>XSAVKAARYGKDNVRVYKVHKDEKTGVQTVYEMTVCVLLEGEIETSYTKADNSVIVATDSIKNTIYITAKQNPVTPPELFGSILGTHFIEKYNHIHAAHVNIVCHRWTRMDIDGKPHPHSFIRDSEEKRNVQVDVVEGKGIDIKSSLSG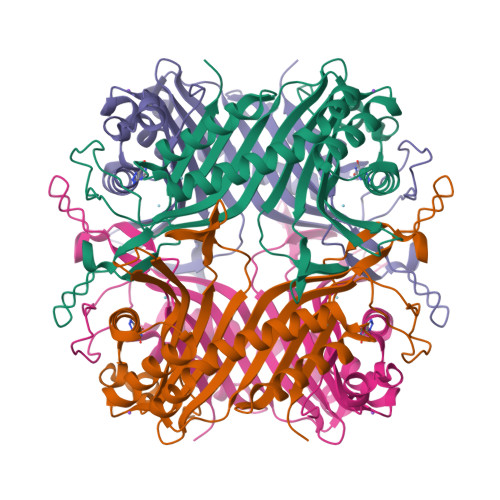LTVLKSTNSQFWGFLRDEYTTLKETWDRILSTDVDATWQWKNFSGLQEVRSHVPKFDATWATAREVTLKTFAEDNSASVQATMYKMAEQILARQQLIETVEYSLPNKHYFEIDLSWHKGLQNTGKNAEVFAPQSDPNGLIKCTVGRS[2x]> MENSLFNQEVQIPLTESYCGPCPK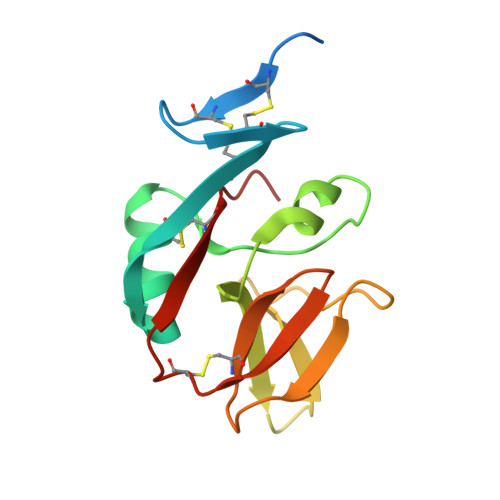NWICYKNNCYQFFDESKNWYESQASCMSQNASLLKVYSKEDQDLLKLVKSYHWMGLVHIPTNGSWQWEDGSILSPNLLTIIEMQKGDCALYASSFKGYIENCSTPNTYICMQRTV(2R)-2-hydroxypentanedioic acid | C5 H8 O5 | 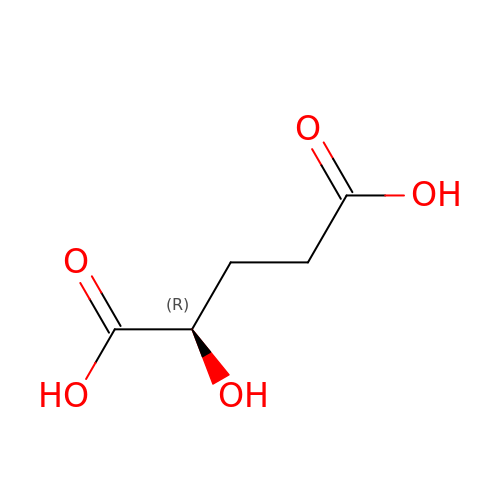HWXBTNAVRSUOJR-GSVOUGTGSA-N>[2x]ASRLERVY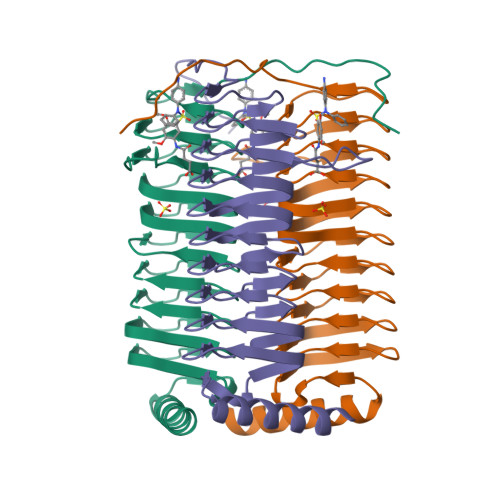QSEQAEKLLLAGVMLRDPARFDLRGTLTHGRDVEIDTNVIIEGNVTLGHRVKIGTGCVIKNSVIGDDCEISPYTVVEDANLAAACTIGPFARLRPGAELLEGAHVGNFVEMKKARLGKGSKAGHLTYLGDAEIGDNVNIGAGTITCNYDGANKFKTIIGDDVFVGSDTQLVAPVTVGKGATIAAGTTVTRNVGENALAISRVPQTQKEGWRRPA> TLPSALLFDCDGVLVDTEKDGHRISFNDTFKERDLNVTWDVD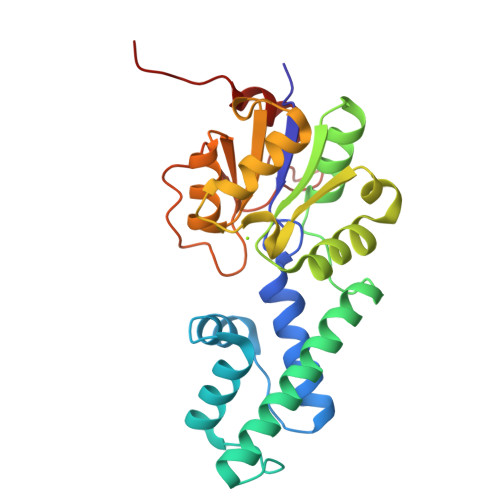LYGELLKIGGGKERMTAYFNKVGWPEKAPKDEAERKEFIAGLHKQKTELFMVLIEKKLLPLRPGVAKLVDQALTNGVKVAVCSTSNEKAVSAIVSCLLGPERAEKIKIFAGDVVPKKKPDPAIYNLAAETLGVDPSKCVVVEDSAIGLAAAKAAGMTCIVTKSGYTADEDFENADAVFDCIGDPPEERFDLAFCGSLLRKQFVS>MPRKKDQVTKNDDGNQTSDVQTQDFKTAVQPDTNTAQLIKTYSNPKQRGDKGEIIYDGGLSSKLADVVDKTTEPHNADGAVKDGRIAPVKLDLEKQKLDKLKLFETSPFDPLTIKNNQDVVDKLYATQSSSIQEVVPTKTFATELQFGVTSEDMAKIYGAVAAVSKNVNSSVTYEVKRGTHELIKVPTIPHNLVLIQSDNGKHALIKEDLGQWPVETGISLVNQAGVFAVQLANKLGIDKPFVLDAGSNYFTDTSFIDTRKYCTDGLSPREIQKALNRQRAYYDRPELTISENKTLLSQSIIYPDADGNDVSIIFSGAMSHAIFTYAQSQWNKNIIKLDDYIREITLTVPKQYRPRRFKEIEHTHGYVYRELNQGSLLPLVDANLKESSSYYFKKLMSSISNVPVDARTLQSATAALAADTGQAVNRAQHVSMLTNRLTTANAPTVRAITVLTCMFKQFRIGMTYALDPNIMDVAAATCMLLFRPAQSISDEQYRYCLQTMAVFLTNTTYDIVNNDTIDVLKMKLRNQGWPFVERYNAVEIDMSVEPLRSPGQVGRYYNPFNIDPLTKKHVEDRLEEFINQVQVGRFRNASGNAVGTTLAAFLRACRDKTSANWRGYSVLVSRYRSLIPNELFESLRNISGEYNINPQDEHSFFFALAQINADDEFIGAIDKESAEYLDEYATLARDISNSLTLVKAAFGPLERTSGSIINHANNLNKVINHVFADKPLISETMLKILTIDGTTGKDGYRNWLDKLVGHNYPVYVEPVVNIMNFISARFVADSSYFGYTNEIMIMPNHINVPVDDRFGFRDSPFCTSLPRTIMGNDVRRISYNVFSMMEDIDDVISEGFILYDAYFNFSYDIMTTDGVTRLKEDILIVTDTGNDIKPIHFYIYFENRNDKKLRYESKMNVSYRLYIKTPACLLPLSDYMRAQHDYVSPSSSRVYIKDPAVVYTRS[2x];>MANRATSAFLDNPHPVGVNYVDEGSRQFVAVAELLASKLIDSSRESDESNSDVPFVQAYSKFADDNPRHLRVKTGGKMANALTNVIRSYYSINAPAIVPQVEIDRLASKATVSGDMYNSYAIFNSVPIVEVLSPARTTVSIVGSDRADVTMLNTGAGAANITFNFGQIAETVILKGSVPFQLARLNQPMPAARFTYKLRPLDGPFIVVLPVGNPLVISATAATRIQVPLAFNKALVESGFQTAMNDGLFDIQNVNYYSSFDEFIISQYHAQDGINRVSTCVILGLALQAYDQMRRALPVRRV[13x];>[2x]MDVLSKGSLKELLAHLEKTPLEEAISYRIGTVPYQNVLISRNEYYNQLYPDTTSLIDGVSREGQRNVNGLIMSIISYVVSGSGHYIPNIGFMLLRRSILDILTKHDTGLVTNNLNYGIIARNLTVSKMNCEQRKRMLICFKLLAYKDGNQNDYEIYLNQNIPLKQIAPNFIPGDMRTVIHNQDQLAIVGIPAYRLTQSTELSIRDDNAKSYKLGYVDWYNSNSFLRERSEFNLIRLKDRDTKYGKLNGW;>[6x]MAWVTQAYSSGLSQNSIISLTGNDRTVADGTFNSMIMPRAVIANEREHFMKTRIDKIEHDLNRSAKQEMMDRQSLAEDYNALNLAVGQEIKLDIATQHQLNRLGSAMYKADHERETELTDLINRIRENEVTVNGILENQKAITAAERADLLLEVVASTAKSVSAAGRAAADGSGVVPVFGPSVANGIKVGIDIADSVAEAAIAVKESGIITQLNDVYHAFQSVHVAPNDVIKPAAVVAGTSTELIGNLQAIYSRLRSHSDIGFKKATVGDVIPNSYMIKPVNSTEYASWQLYVIHPVQGSLGLVVQLMGDALTYNVFAQYGNTSASEFGKTVLTGGATNTALEGTKVKFQTKVTAQQALALTMALKDAASMLSQGELIGYFEQYINLALEPDNLSLQDNMHKYHHLLTSQNSPIDWNYHDEEMHKWLDSRKTTNYDAMQKKDGTVIADIHIPKVFNDLRNTTLHCKLEGKQTIAGYTVYEYLIGPWAHYGDIDYSVVVDTLNEETKWYCEVIGIDGHLLIEKSVQHKPEKILELTVNDSGVTSFNGRNHDRLKLKVYVKDSLSVKVFRNWIGINAPRVKTKMFNDHIGVKYDYSHFDKNISPAHLTLTDLGWHTWDQYNAGNWTNIKP;>[6x]MLSETELRALKKLSTTTSRVVGDSTLALPSNVKLSKGEVEKIAVTKKEMFDELAQCNLPTIELITREHTFNGDVIRFAAWLFLMNGQKLMIANNVAVRMGMQYATNLAGNNVKITYVTSNNVVKLGHIAAGVLANPYSNKGSGLFITYEYNLISNLIETGKVCVLFIT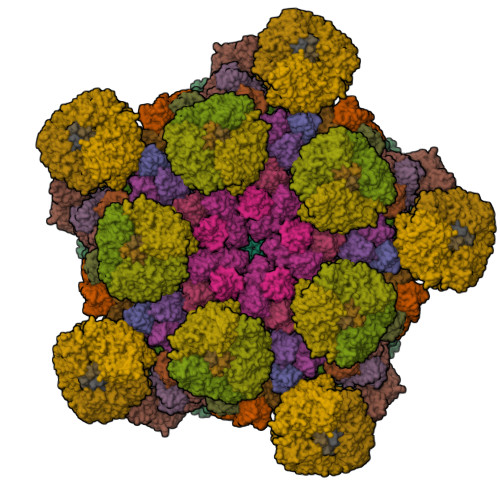SLSTTASSTNSFAYSTCSVPIENWDFNMIKLTAETSCASLTAMTNLVNSLVPGERTRPVGLYVDIPGVTVTTSASSGSLPLTTIPAVTPLIFSAYTKQVEEVGVINTLYALSYLP>MEWSWVFLFFLSVTTGVHSLIRIPLRKFTSIRRTMTEVGGSVEDLILKGPITKYSMQSSPRTKEPVSELLKNYLDAQYYGEIGIGTPPQCFTVVFDTGSSNLWVPSIHCKLLDIACWVHHKYNSDKSSTYVKNGTSFDIHYGSGSLSGYLSQDTVSVPCKSDLGGIKVEKQIFGEATKQPGVVFIAAKFDGILGMGYPFISVNNVLPVFDNLMKQKLVEKNIFSFYLNRDPTGQPGGELMLGGTDSRYYHGELSYLNVTRKAYWQVHMDQLEVGSELTLCKGGCEAIVDTGTSLLVGPVDEVKELQKAIGAVPLIQGEYMIPCEKVSSLPIITFKLGGQNYELHPEKYILKVSQAG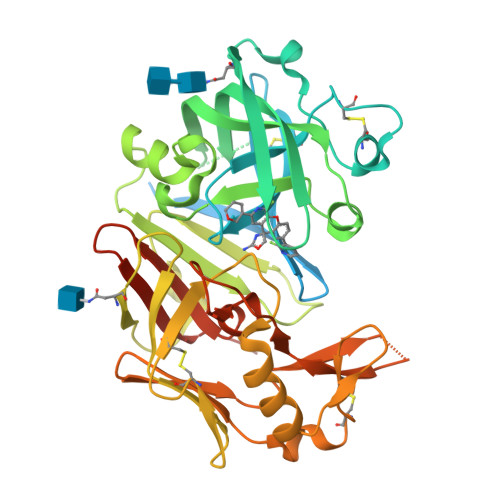KTICLSGFMGMDIPPPSGPLWILGDVFIGCYYTVFDREYNRVGFAKAATLDEVDHHHHHHHHHH[2x]EccC, the motor subunit of T7SS, is essential to assemble a stable membrane complex for the secretion process. It contains a two-pass transmembrane domain, an unknown function domain (DUF), and three Fts-SpoIIIE-like ATPase domains (ATPase1, ATPase2, and ATPase3). In this study, we have provided high-resolution crystal structures of ATPase3 domains of EccC proteins from Mtb, all in complex with ATP. In our structures, ATP and a magnesium ion bind to the nucleotide-binding site in a similar manner.

To explain structure-function differences amongst EccC-ATPase3 domains, the crystal structures of Mtb ATPase3 from ESX-2, -3, -5 were determined at 2.20 Å, 1.97 Å and 2.00 Å resolution, respectively. Though the sequence identities are only 20%~30% amongst the four ATPase3 domains, their atomic structures can be superimposed and have r.m.s.d. values in the range 0.99~2.02 Å by comparing Cɑ atom pairs. Here, our structural data showed that the recognition pocket in each EccC-ATPase3 is different. The signal binding pocket of MtEccC3-ATPase3 is much wider than MtEccCb1-ATPase3; the pocket of MtEccC5-ATPase3 is much flatter while MtEccC2-ATPase3 has a shallow recognition pocket. The different shapes and compositions of signal recognition pockets further imply that different T7SS subtypes could specifically recognize individual substrates.

> MKYLLPTAAAGLLLLAAQPAMAMDSSGLEVLFQGPGSPGMAAPPVRLLPTNLAPHAVGELYRGPDQLVIGQREEDLAPVILDLAANPLLMVFGDARSGKTTLLRHIIRTVREHSTADRVAFTVLDRRLHLVDEPLFPDNEYTANIDRIIPAMLGLANLIEARRPPAGMSAAELSRWTFAGHTHYLIIDDVDQVPDSPAMTGPYIGQRPWTPLIGLLAQAGDLGLRVIVTGRATGSAHLLMTSPLLRRFNDLQATTLMLAGNPADSGKIRGERFARLPAGRAILLTDSDSPTYVQLINPLVDAAAVSGETQQKGSQSLEHHHHHH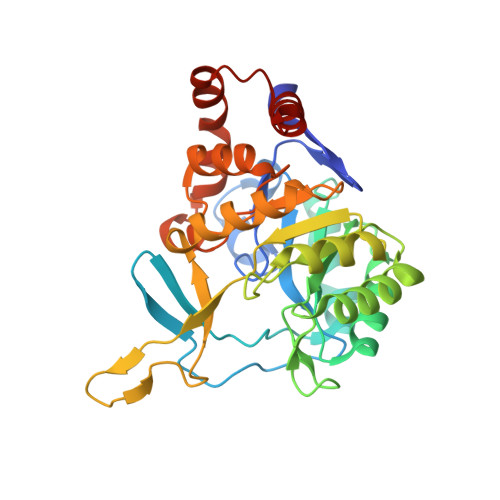> MTENNRLSVKLPGLDLKNPIIPASGCFGFGEEYAKYYDLNKLGSIMVKATTLHPRFGNPTPRVAETASGMLNAIGLQNPGLEVIMTEKLPWLNENFPELPIIANVAGSEEADYVAVCAKIGDAANVKAIELNISCPNVKHGGQAFGTDPEVAAALVKACKAVSKVPLYVKLSPNVTDIVPIAKAVEAAGADGLTMINTLMGVRFDLKTRQPILANITGGLSGPAIKPVALKLIHQVAQDVDIPIIGMGGVANAQDVLEMYMAGASAVAVGTANFADPFVCPKIIDKLPELMDQYRIESLESLIQEVKEGKK> GSSHHHHHHLEVLFQGPAELEHLAQNISKSHLETCQYLREELQQITWQTFLQEEIENYQNKQREVMWQLCAIKITEAIQYVVEFAKRIDGFMELCQNDQIVLLKAGSLEVVFIRMCRAFDSQNNTVYFDGKYASPDVFKSLGCEDFISFVFEFGKSLCSMHLTEDEIALFSAFVLMSADRSWLQEKVKIEKLQQKIQLALQHVLQKNHREDGILTKLICKVSTLRALCGRHTEKLMAFKAIYPDIVRLHFPPLYKELFTSEFE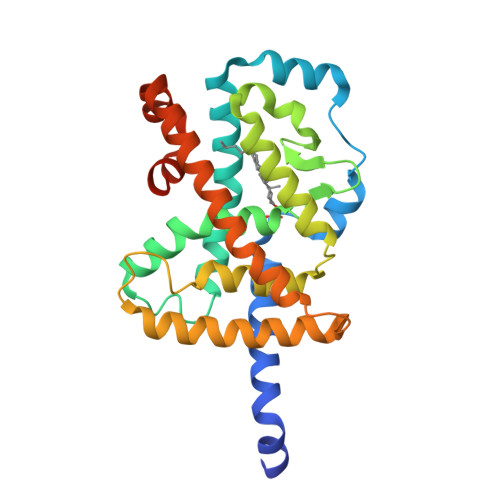PAMQIDG>[2x]MTNTTLDNNALDNNKLSPWPWQVDEAAISFDIESLGKKLKDLNQACYLINHAEKGLGIAQSAEVVGLAEPNNGLHPVSAFAPALGTQSLGDSNFRRVHGVKYAYYAGAMANGIASEELVIALGQAGILCSFGAAGLIPSRVEAAIKRIQAALPNGPYAFNLIHSPSEQALERGS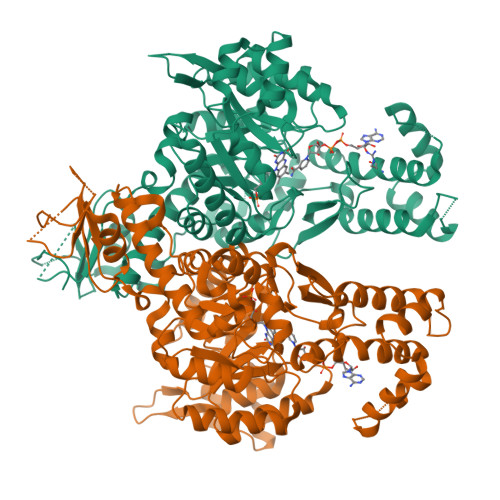VELFLKHQVRTVEASAFLGLTPQIVYYRAAGLSRDASGEIVIGNKVIAKISRTEVATKFMEPAPVKILQQLVNEGLISEDQMLMAQSVPMADDITAEADSGGHTDNRPLVTLLPTILALKDTIQAKYQYKTPIRVGAGGGIGTPDAALATFNMGAAYIVTGSINQACVEAGASEHTRKLLATTEMADVTMAPAADMFEMGVKLQVVKRGTLFPMRANKLYEIYTRYDSIEAIPAEERQKLEEQVFRASLDEIWAGTVAHFNERDPKQIERALDNPKRKMALIFRWYLGLSSRWSNTGEVGREMDYQIWAGPALGAFNAWAKGSYLDDYRERNAVDLAKHLMQGAAYQARINLLLSQGVSIPVSLQRWKPLQRC> MQKTLEVWIMPNSPQPAEDFKALVAPFEKAHGVEVKVTVLDWGVAWTKITTAATSGVGPDLTQLGTTWVGAISA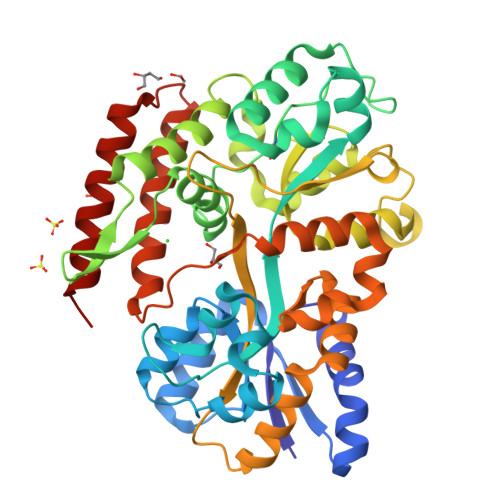MGVLEPVDDVLEALGGEKAYLPAVWRTTRLEGARQATAVPWFSELRAFYYRTDALKAAGVNPAEMFASWQGFEAGLARLKASSFRDPETKAPLAPLCTPGKNSWDVLHNAAPWIWGAGGEIVRQAGGRWQSALNSPESLEGLYFFLSLAQKGYVPAESLEKNTAQIEADFQAGKCAVFASGPWMIQRAQVPEAKGGFAERTAAKNLGVAPYPAGPKGRYTFFGGSNLALFNFSKNKPLAKELLKYLGGPEAQVRYAQMTGMLPALRSAWSDPSFQQNPLLRTFIQAAQFGRTYPSLAGWGGVENLAVQHLGMAWDLVAQGRLTREALKDLMDKASAAINQALRHHHHHH> QENQDGRYSLTYIYTGLSKHVEDVPAFQALGSLNDLQFFRYNSKDRKSQPMGLWRQVEGMEDWKQDSQLQKAREDIFMETLKDIVEYYKDSTGSHVL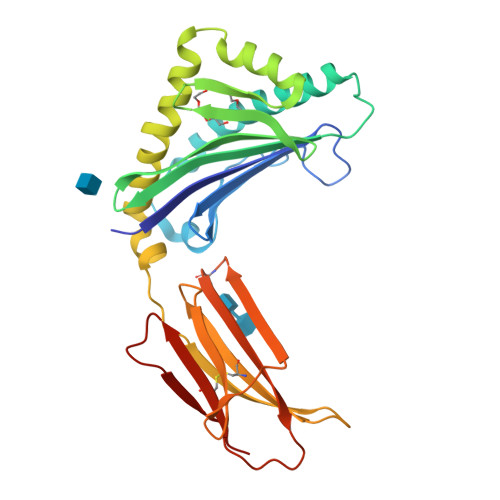QGRFGCEIENNRSSGAFWKYYYDGKDYIEFNKEIPAWVPFDPAAQITKQKWEAEPVYVQRAKAYLEEECPATLRKYLKYSKNILDRQDPPSVVVTSHQAPGEKKKLKCLAYDFYPGKIDVHWTRAGEVQEPELRGDVLHNGNGTYQSWVVVAVPPQDTAPYSCHVQHSSLAQPLVVPWEAS>MKKIIETQRAPGAIGPYVQGVDLGSMVF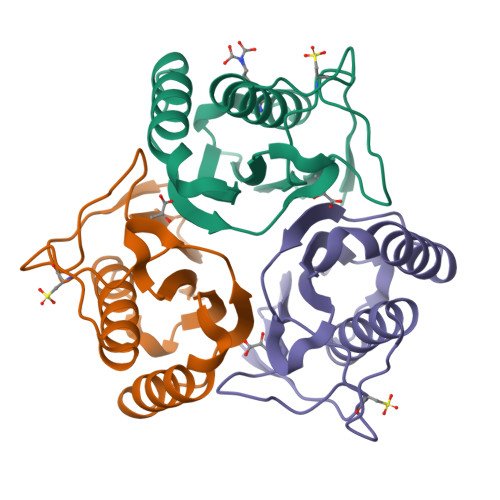TSGQIPVCPQTGEIPADVQDQARLSLENVKAIVVAAGLSVGDIIKMTVFITDLNDFATINEVYKQFFDEHQATYPTRSCVQVARLPKDVKLEIEAIAVRSA[3x]> MGSSHHHHHHSQDPGGTGHLISSTGALGSR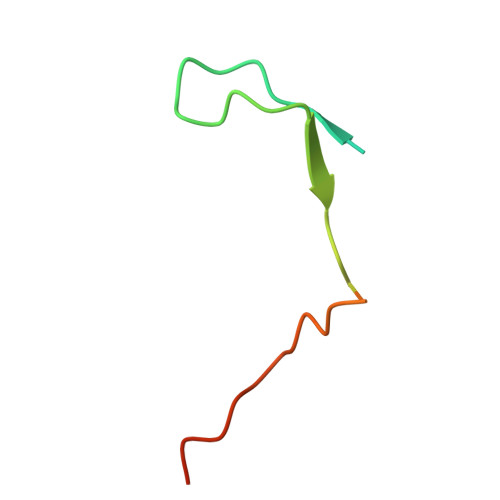SLFSPLRNSMADSVDSRDIPGLPTNPSRLAAAT>[2x]SMNWDDHAIIIFGYPETIANSIILHFANFGEILEDFRVIKDFKKLNSKNMSKSPSLT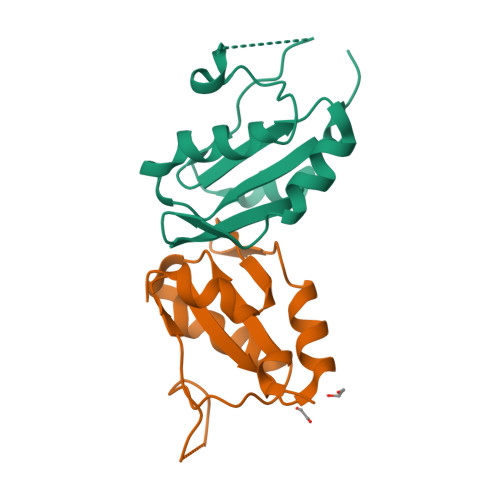AQKYPIYTGDGWVKLTYKSELSKSRALQENGIIMNGTLIGCVSYSPAALKQLAS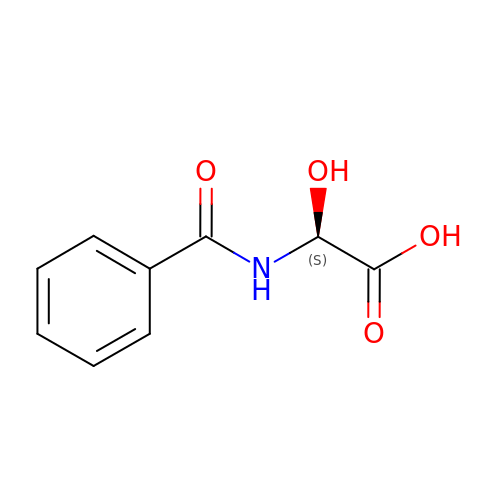(2S)-hydroxy[(phenylcarbonyl)amino]ethanoic acid | C9 H9 N O4 | GCWCVCCEIQXUQU-QMMMGPOBSA-N> MGHHHHHHPPFEKNFYNEHEEITNLTPQQLIDLRHKLNLRVSGAAPPRPGSSFAHFGFDEQLMHQIRKSEYTQPTPIQCQGVPVALSGRDMIGIAKTGSGKTAAFIWPMLIHIMDQKELEPGDGPIAVIVCPTRELCQQIHAECKRFGKAYNLRSVAVYGGGSMWEQAKALQEGAEIVVCTPGRLIDHVKKKATNLQRVSYLVFDEADRMFDMGFEYQVRSIASHVRPDRQTLLFSATFRKKIEKLARDILIDPIRVVQGDIGEANEDVTQIVEILHSGPSKWNWLTRRLVEFTSSGSVLLFVTKKANAEELANNLKQEGHNLGLLHGDMDQSERNKVISDFKKKDIPVLVATDVAARGLDIPSIKTVINYDVARDIDTHTHRIGRTGRAGEKGVAYTL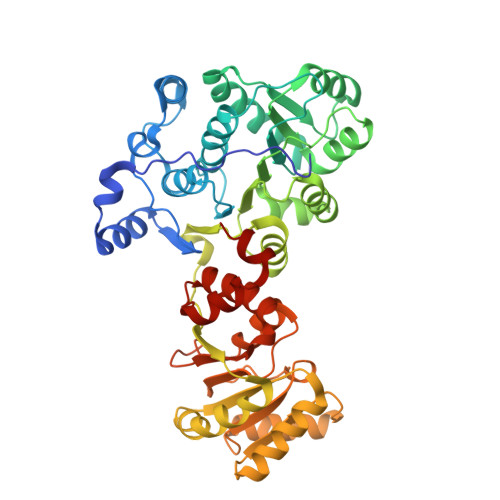LTPKDSNFAGDLVRNLEGANQHVSKELLDLAMQNAWFRKSRFKGG>MLRTILDAPQRLLKEGRASRQLVLVVVFVALLLDNMLFTVVVPIVPTFLYDMEFKEVNSSLHLGHAGSNCLQGTGFLEEEITRVGVLFASKAVMQLLVNPFVGPLTNRIGYHIPMFAGFVIMFLSTVMFAFSGTYTLLFVARTLQGIGSSFSSVAGLGMLASVYTDDHERGRAMGTALGGLALGLLVGAPFGSVMYEFVGKSAPFLILAFLALLDGALQLCILQPSKVSPESAKGTPLFMLLKDPYILVAAGSICFANMGVAILEPTLPIWMMQTMCSPKWQLGLAFLPASVSYLIGTNLFGVLANKMGRWLCSLIGMLVVGTSLLCVPLAHNIFGLIGPNAGLGLAIGMVDSSMMPIMGHLVDLRHTSVYGSVYAIADVAFCMGFAIGPSTGGAIVKAIGFPWLMVITGVINIVYAPLCYYLRSPPAKEEKLAILSQDCPM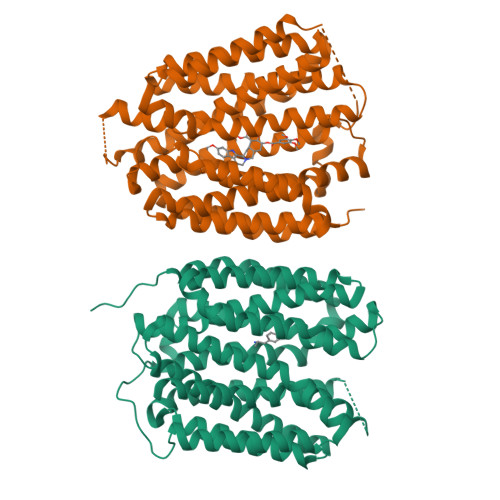ETRMYATQKPTKEFPLGEDSDEEPDHEE[2x]>MSYTVGTYLAERLVQIGLKHHFAVAGDYNLVLLDNLLLNKNMEQVYCCNELNCGFSAEGYARAKGAAAAVVTYSVGALSAFDAIGGAYAENLPVILISGAPNNNDHAAGHVLHHALGKTDYHYQLEMAKNITAAAEAIYTPEEAPAKIDHVIKTALREKKPVYLEIACNIASMPCAAPGPASALFNDEASDEASLNAAVEETLKFIANRDKVAVLVGSKLRAAGAEEAAVK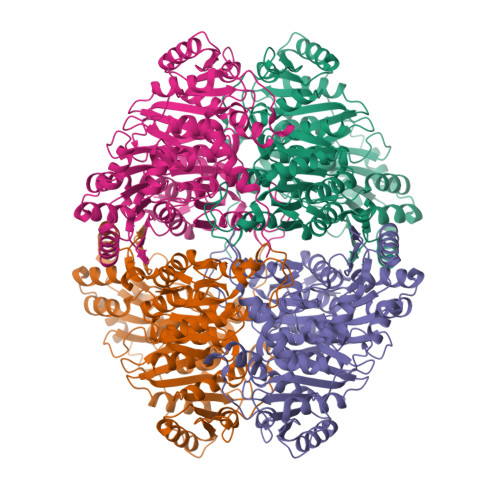FADALGGAVATMAAAKSFFPEENPHYIGTSWGEVSYPGVEKTMKEADAVIALAPVFNDYSTTGWTDIPDPKKLVLAEPRSVVVNGIRFPSVHLKDYLTRLAQKVSKKTGALDFFKSLNAGELKKAAPADPSAPLVNAEIARQVEALLTPNTTVIAETGDSWFNAQRMKLPNGARVEYEMQWGHIGWSVPAAFGYAVGAPERRNILMVGDGSFQLTAQEVAQMVRLKLPVIIFLINNYGYTIEVMIHDGPYNNIKNWDYAGLMEVFNGNGGYDSGAGKGLKAKTGGELAEAIKVALANTDGPTLIECFIGREDCTEELVKWGKRVAAANSRKPVNKLL[8x]Spermidine/spermine N-acetyltransferases (SSATs) are catabolic enzymes that acetylate polyamines and are critical for maintaining intracellular polyamine homeostasis. SpeG is an SSAT protein found in a variety of bacteria, including the human pathogen Vibrio cholerae. This protein adopts a dodecameric structure and contains an allosteric site, making it unique compared to other SSATs. The allosteric site is located between monomers that form the hexamers of the dodecamer, and some evidence has been provided that shows when polyamine binds to these sites, the dodecamer tightens.

R1C1 replaces all residues of this region with the hSSAT1 protein sequence, R1C2 replaces the first half of the residues, R1C3 replaces the first three quarters of the residues, and R1C4 replaces the latter half of the residues of this region. All substituted residues of the VcSpeG protein sequences of these constructs were ordered in the structures, with the exception of R1C3, which had ARYEYME residues of the substitution that were disordered. However, the R1C3 crystal structure had a disordered region (K23-Q34) which contributed to the higher rmsd value for the overlaid apo-structure and homology model. Our analysis of the apo-crystal structures and corresponding homology models of the monomer showed good root mean square deviations (rmsd) between the two (R1C2 rmsd 1.45 Å, R3C1 rmsd 1.17 Å, R3C4 rmsd 1.01 Å, R3C5 rmsd 1.25 Å, and R3C7 rmsd 1.20 Å), with the exception of R1C3 which had an rmsd of 4.33 Å. Alternatively, when the first three quarters of the loop or latter half of the loop residues were substituted (R1C3 and R1C4, respectively), the enzyme activity decreased by 52-fold for R1C3 and no activity was detected for the R1C4 construct. A more drastic decrease in catalytic efficiency was observed for the R1C1 construct (two orders of magnitude compared to WT) compared to the R1C3 construct (one order of magnitude compared to WT). Based on the kinetic results, it became clear that the region of the allosteric loop that was critical for activity was between residues 31–34 (WFEE). The R1C1, R1C3, and R1C4 constructs all have MEEQ in place of WFEE, which would disrupt these interactions and may explain the reduced activity of these constructs. The investigation of alterations to Region 1 of the VcSpeG protein (R1C1-R1C4) showed we could replace residues in the first half of the allosteric loop (R1C2) and retain moderate activity, but exchanging residues in either the second half of the loop (R1C4), the first three quarters of the loop (R1C3) or the entire loop (R1C1) caused the enzyme to be inactive. Therefore, residues within the WFEE portion of the allosteric loop are critical for activity, but we do not know whether all residues or only a subset of these four residues are required for activity toward spm for the VcSpeG enzyme.

>[3x]MNSQLTLRALERGDLRFIHNLNKELARYEYMEEQPYESFDELEELYNKHIHDNAERRFVVEDAQKNLIGLVELIEINYIHRSAEFQIIIAPEHQGKGFARTLINRALDYSFTILNLHKIYLHVAVENPKAVHLYEECGFVEEGHLVEEFFINGRYQDVKRMYILQSKYLNRSE> HMLDPEEIRKRLEHTERQFRNRRK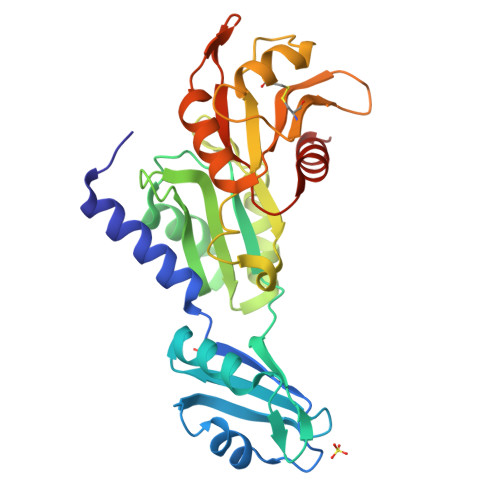ILIRGLPGDVTNQEVHDLLSDYELKYCFVDKYKGTAFVTLLNGEQAEAAINAFHQSRLRERELSVQLQPTDALLCVANLPPSLTQQQFEELVRPFGSLERCFLVYSERTGQSKGYGFAEYMKKDSAARAKSDLLGKPLGPRTLYVHWTDAGQLTPALLHSRCLCVDRLPPGFNDVDALCRALSAVHSPTFCQLACGQDGQLKGFAVLEYETAEMAEEAQQQADGLSLGGSHLRVSFCAPGPPGRSMLAALIAAQATALNR> TSDLIPAPPLSKVPLQQNFQDNQFQGKWYVVGLAGNAILREDKDPQKMYATIYEEKEDASYNVTSVLFRKKKCDYAIRTFVP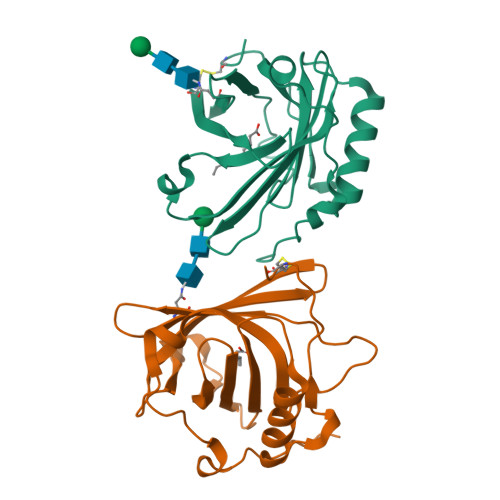GCQPGEFTLGNIKSYPGLTSYLVRVVSTNYNQHAMVFFKKVSQNREYFKITLYGRTKELTSELKNNFIRFSKSLGLPENHIVFPVPIDQCID>[3x]MAFSGSQAPYLSPAVPFSGTIQGGLQDGLQITVNGTVLSSSGTRFAVN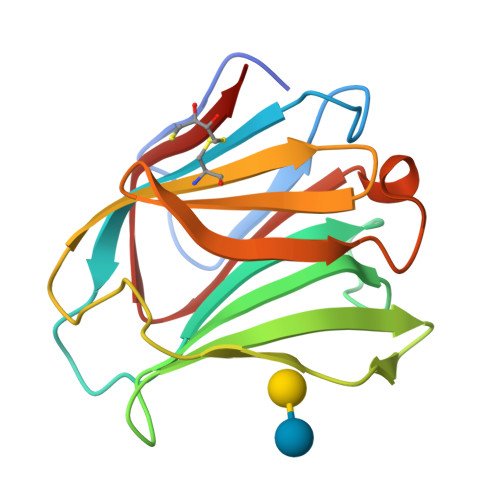FQTGFSGNDIAFHFNPRFEDGGYVVCNTRQNGSWGPEERKTHMPFQKGMPFDLCFLVQSSDFKVMVNGILFVQYFHRVPFHRVDTISVNGSVQLSYISFQ>MRNKIFISHATPDDNDFTRWLALKLIGLGYEVWCDILFLDKGVDFWSNIEKVIREDTCKFLLVSSSYSNQREGVLKELAVAAKVKKQLKDDKFIIPLAIDEQLSYDDINIDIVRLNAIDFKMSWARGLKDILEAFEKQKVPKEVADASKSNLLYQQIFLHDKSVIEKEEIYDSNWLSILSFPEELRFHEYNWMLPKRFDVRELTFPAVRYKNYLCTFAWAYDFTYHLPKTETYHKSKTIRIPTEEILSGSYDSNFIRNAECKRLIVQLLNKAFELRMKDKEVQEYEMSNKTAYWLEKGKLEKDKFEKTMLVGKQKDKNWHFAISGASKLYPFPVLMISSHIFFTADGKKLIDSSSVQHSSRRRQGKNWWNNTWRTKLLAFIKYLSDDDTSFYLEMGSEEKVFVSNEPVKFKGNVSYNIPEKNTLEEEAELSGFNQGEDIEELEELIENLEAE[2x];>MKELIYIEEPKILFAHGQKCTDARDGLALFGPLNNLYGIKSGVIGTKQGLKIFRDYLDHIQKPIYNSNSITRPMFPGFEAVFDCKWESTGITFKEVTNEDIGKFLYNSSTHKRTYDLVSLFIDKIISANKNEDENVDVWFVIVPDEIYKYCRPNSVLPKEMVQTKALMSKSKAKSFRYEPSLFPDINIELKEQEKEAETYNYDAQFHDQFKARLLKHTIPTQIFRESTLAWRDFKNAFGLPIRDFSKIEGHLAWTISTAAFYKAGGKPWKLSDVRNGVCYLGLVYKKVEKSKNPRNACC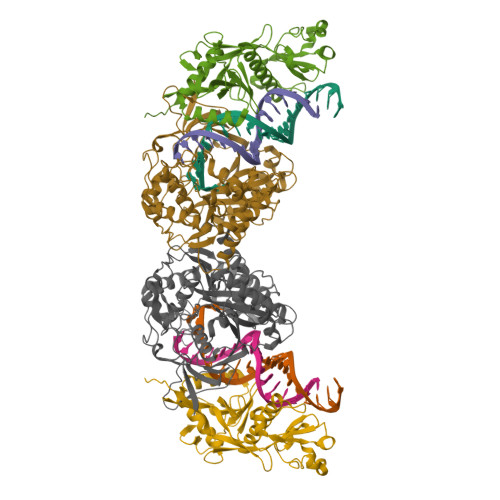AAQMFLDNGDGTVFKGEVGPWYNPKNGQYHLEPKEAKALLSQSLQSYKEQIGEYPKEVFIHAKTRFNHQEWDAFLEVTPKETNLVGVTISKTKPLKLYKTEGDYTILRGNAYVVNERSAFLWTVGYVPKIQTALSMEVPNPLFIEINKGEADIKQVLKDILSLTKLNYNACIFADGEPVTLRFADKIGEILTASTDIKTPPLAFKYYI[2x]> TQAKAKHADVPVNLYRPNAPFIGKVISNEPLVKEGGIGIVQHIKFDLTGGNLKYIEGQSIGIIPPGVDKNGKPEKLRLYSIASTRHGDDVDDKTISLCVRQLEYKHPE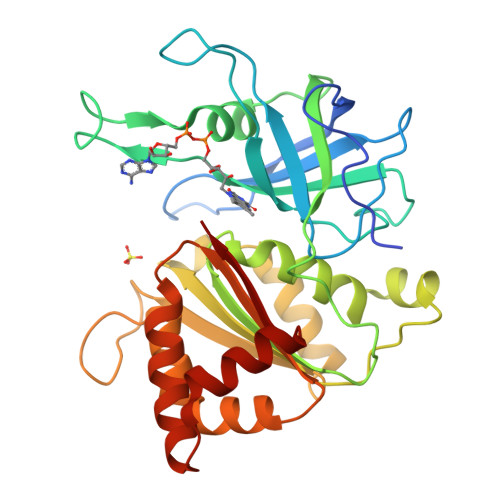SGETVYGVCSTYLTHIEPGSEVKITGPVGKEMLLPDDPEANVIMLAGGTGITPMRTYLWRMFKDAERAANPEYQFKGFSWLVFGVPTTPNILYKEELEEIQQKYPDNFRLTYAISREQKNPQGGRMYIQDRVAEHADQLWQLIKNQKTHTYICGLRGMEEGIDAALSAAAAKEGVTWSDYQKDLKKAGRWHVETY>GSHMLEMRIGHGFDVHAFGGEGPIIIGGVRIPYEKGLLAHSDGDVALHALTDALLGAAALGDIGKLFPDTDPAFKGADSRELLREAWRRIQAKGYTLGNVDVTIIAQAPKMLPHIPQMRVFIAEDLGCHMDDVN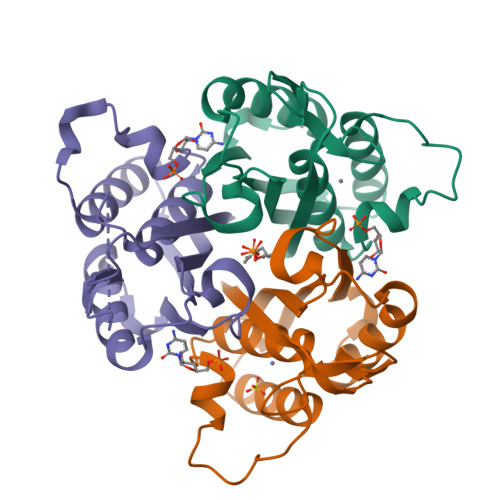VKATTTEKLGFTGRGEGIACEAVALLIKATK[6x]> AATTGYDAVDDLLHYHERGNGIQI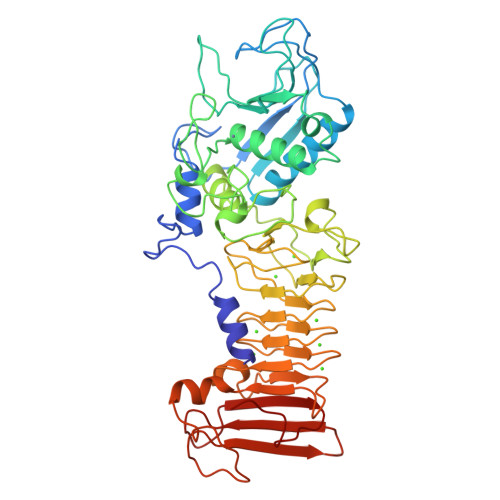NGKDSFSNEQAGLFITRENQTWNGYKVFGQPVKLTFSFPDYKFSSTNVAGDTGLSKFSAEQQQQAKLSLQSWADVANITFTEVAAGQKANITFGNYSQDRPGHYDYGTQAYAFLPNTIWQGQDLGGQTWYNVNQSNVKHPATEDYGRQTFTHEIGHALGLSHPGDYNAGEGDPTYADVTYAEDTRQFSLMSYWSETNTGGDNGGHYAAAPLLDDIAAIQHLYGANLSTRTGDTVYGFNSNTGRDFLSTTSNSQKVIFAAWDAGGNDTFDFSGYTANQRINLNEKSFSDVGGLKGNVSIAAGVTIENAIGGSGNDVIVGNAANNVLKGGAGNDVLFGGGGADELWGGAGKDIFVFSAASDSAPGASDWIRDFQKGIDKIDLSFFDKEANSSSFIHFVDHFSGTAGEALLSYNASSNVTDLSVNIGGHAAPDFLVKIVGQVDVATDFIV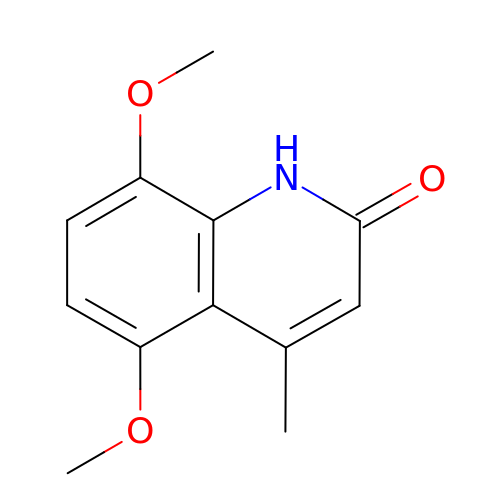5,8-dimethoxy-4-methylquinolin-2(1H)-one | C12 H13 N O3 | BUHDAIGNGIXQJO-UHFFFAOYSA-N> MGNCLDSSAKVDNSNHSPHANSASSGSKVSSKTSRSTGPSGLSTTSYSTDSSFGPLPTLRTEGEILSSPNLKAFTFNELKNATKNFRQDNLLGEGGFGCVFKGWIDQTSLTASRPGSGIVVAVKQLKPEGFQGHKEWLTEVNYLGQLSHPNLVLLVGYCAEGENRLLVYEFMPKGSLENHLFRRGAQPLTWAIRMKVAVGAAKGLTFLHEAKSQVIYRDFKAANILLDADFNAKLSDFGLAKAGPTGDNTHVSTKVIGTHGYAAPEYVATGRLTAKSDVYSFGVVLLELISGRRAMDNSNGGNEYSLVDWATPYLGDKRKLFRIMDTKLGGQYPQKGAFTAANLALQCLNPDAKLRPKMSEVLVTLEQLESVAKPGTKHTQMESPRFHHSSVMQKSPVRYSHDRPLLHMTPGASPLPSYTQSPRVR;> MKKQYLKSGSGTRKEKDKAKRWFLDNGSIFLRELVADCNGKSIPIRSFSPEQILKATNNFDSSCFVSQDVYYKWYRGEIEDRSYMIKRFSEDEITGKRHRVKEVYNDIVLSARMSNHSNFLQLLGCCLEFPFPVLVFEFAEHGAMNQRGGVIVNGEESLLPWSVRLKIGKEIANAVTYLHTAFPKIIIHRDVKPMHVFLDKNWTAKLSDLSFSISLPEGKSRIEAEWVLGTFGYIDPLYHKTCFVTEYTDVYSFGICLLVIITGKPAIMTISDGDLQGILSLVRELCENGKLDEVIDPRLMKDITSGQRLQVEACVVLALRCCKERDEDRPKMIQVAKELKQIEASLKNSS;>MVDAVVTVFLEKTLNILEEKGRTVSDYRKQLEDLQSELKYMQSFLKDAERQKRTNETLRTLVADLRELVYEAEDILVDCQLADGDDGNEQRSSNAWLSRLHPARVPLQYKKSKRLQEINERITKIKSQVEPYFEFITPSNVGRDNGTDRWSSPVYDHTQVVGLEGDKRKIKEWLFRSNDSQLLIMAFVGMGGLGKTTIAQEVFNDKEIEHRFERRIWVSVSQTFTEEQIMRSILRNLGDASVGDDIGTLLRKIQQYLLGKRYLIVMDDVWDKNLSWWDKIYQGLPRGQGGSVIVTTRSESVAKRVQARDDKTHRPELLSPDNSWLLFCNVAFAANDGTCERPELEDVGKEIVTKCKGLPLTIKAVGGLLLCKDHVYHEWRRIAEHFQDELRGNTSETDNVMSSLQLSYDELPSHLKSCILTLSLYPEDCVIPKQQLV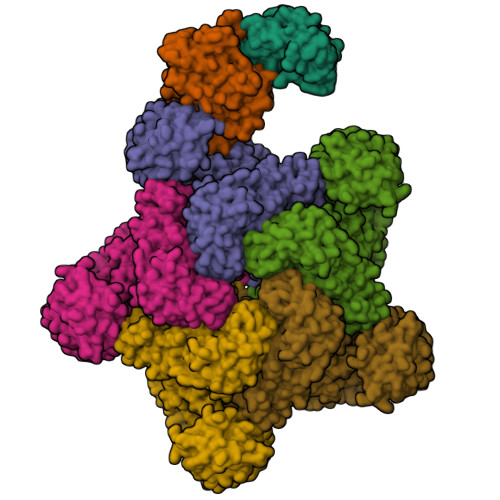HGWIGEGFVMWRNGRSATESGEDCFSGLTNRCLIEVVDKTYSGTIITCKIHDMVRDLVIDIAKKDSFSNPEGLNCRHLGISGNFDEKQIKVNHKLRGVVSTTKTGEVNKLNSDLAKKFTDCKYLRVLDISKSIFDAPLSEILDEIASLQHLACLSLSNTHPLIQFPRSMEDLHNLQILDASYCQNLKQLQPCIVLFKKLLVLDMTNCGSLECFPKGIGSLVKLEVLLGFKPARSNNGCKLSEVKNLTNLRKLGLSLTRGDQIEEEELDSLINLSKLMSISINCYDSYGDDLITKIDALTPPHQLHELSLQFYPGKSSPSWLSPHKLPMLRYMSICSGNLVKMQEPFWGNENTHWRIEGLMLSSLSDLDMDWEVLQQSMPYLRTVTANWCPELESFAIEDVGFRGGVWMKTPLHRT[5x]>[2x]SNAMSKFYQINTTLLESNEAVNKQ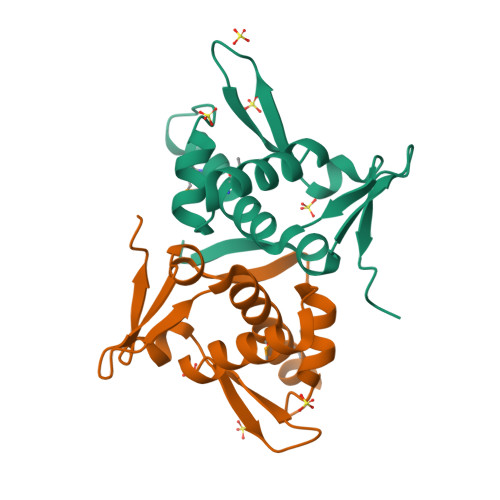TGEVVPLSPETKLVYAYMLNQYRMYRKYGNRRYTESWDKIFTVCCDVAAQKQKRLAKELTTLGLIEVIGNKNAYKVVHSVESIIETWEFTNSKLNT Sorbicillinoids are yellow secondary metabolites synthesized through an elegant combination of enzymatic and spontaneous biochemical processes. The flavin-dependent monooxygenase SorC and oxidase SorD are crucial in this interplay, enabling the generation of a diverse array of functionally complex sorbicillinoids. SorA and SorB work in tandem to synthesize the hexaketide precursor sorbicillin, while SorC and SorD are involved in the subsequent oxidative processes, including dimerization and oxidation reactions.11,12 Specifically, the monooxygenase SorC catalyzes the oxidative dearomatization of sorbicillin to form (S)-sorbicillinol. The oxidase SorD can then use hydrated sorbicillinol and oxidize it to oxosorbicillinol.

SorC crystallized as a monomer, which is consistent with size-exclusion chromatography and mass photometry analyses. The general structure was solved at 1.4 Å, and consists of two domains: a Rossmann fold FAD-binding domain (residues 9–185 and 302–403) containing a binding site for the adenosine diphosphate moiety of FAD, and the catalytic middle domain (residues 186–301) that binds the substrate. In class A flavin-dependent monooxygenases, substrate binding generally initiates flavin reduction by promoting the out conformation of the flavin. The crystal structure of SorC without sorbicillin shows that the oxidized flavin is already in the out conformation. This allows a passage for sorbicillin to enter into the active site. In fact, two poly(ethylene glycol) molecules reside in or near the entry of the active site of SorC. The out positioning of the flavin also generates a cavity close to the cofactor that provides space for the nicotinamide to enter and allow reduction of FAD. Analysis of the environment around FAD revealed that the cofactor is in the out conformation. Trp300, located on the re-face of FAD, forms π–π stacking interactions with the isoalloxazine ring, thereby stabilizing this out conformation. Furthermore, a flexible Arg201 residue provides additional hydrogen-bonding interactions with the O4 and N5 of the isoalloxazine ring. In SorC, the residue Asn331 promotes the FAD out conformational change by forming H-bonding interactions with Gln197.

> MTRSANSPFEVAIVGGGITGLALAVGLLKRNVSFTIYERAENFGELGVGITFTPNAQRAMEALDPCVLQSFTNVASAPSGGTINFVDGVREQGSEDPRTSTAALLFQLHVKGGYKACRRCDFVDQIVQHIPKDCVQYRKWLDSIETDHESGRAVLKFRDGEIAHADVVIGCDGIRSQVRASMFGTDELCPRAQYSHQLGYRGMVPLAQATAVLGPEKTSSAVLHTGPGAFVLTIPLAEVHAMHIEAFIMDKEEWPEVQTSSDSKRYVLPATRNEATKAFAEFGPTVRSAVSMFPEKLEKWAVFDMLEAPVPTFAKGRVCLAGDAAHASTPNQGGGAGFGIEDALVLAEVLAVLAEAPNVSGIVASEALAVYSEVRYERSQWLVRSSRRTGELCTWKDRDWGLAAEELSRDIISRSHQLWDHDTAGMVSDALAILGERVRGADTAF>[2x]GQS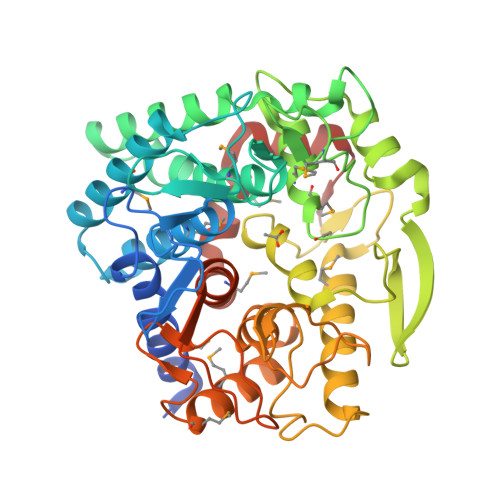CKGKSSSNLTAATDSLSDDALMDTVQRRTFLYFWEGAEPNSGLAPERYHVDGVYPQNDANVVTSGGSGFGIMAILAGIDRGYVTREEGLARMERIVSFLEKADRFHGAYPHWWYGDTGKVKPFGQKDNGGDLVETAFLMQGLLAVHQYYANGNDKEKAIAQRIDRLWREVDWDWYRKGGQNVLYWHWSPTYGWEMDFPIHGYNECMIMYILAAASPTHGVPAAVYHDGWAQNGAIVSPHKVEGIELHLRYQGTEAGPLFWAQYSFLGLDPVGLKDEYCPSYFHEMRNLTLVNRAYCIRNPKHYKGFGPDCWGLTASYSVDGYAAHSPNEQDDKGVISPTAALSSIVYTPEYSLQVMRHLYNMGDKVFGPFGFYDAFSETDNWYPQRYLAIDQGPIAVMIENYRTGLLWKLFMSHPDVQAGLTKLGFNTNKQDVRQQ>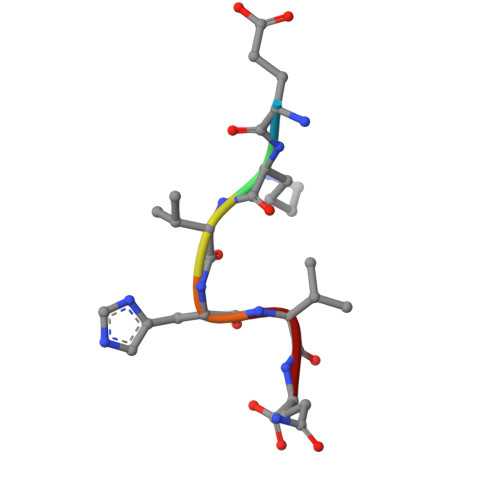 EKVHVQ> GPLGSMSGIALSRLAQERKAWRKDHPFGFVAVPTKNPDGTMNLMNWECAIPGKKGTPWEGGLFKLRMLFKDDYPSSPPKCKFEPPLFHPNVYPSGTVCLSILEEDKDWRPAITIKQILLGIQELLNEPNIQDPAQA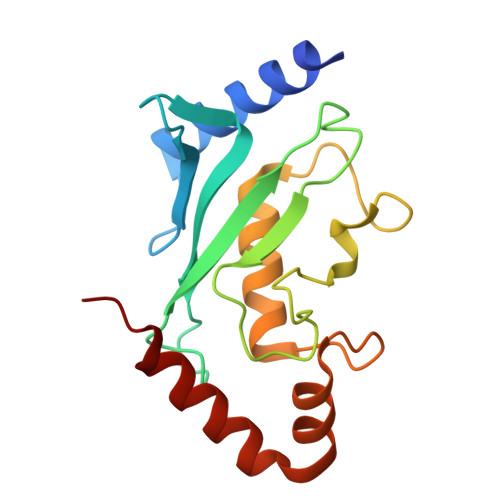EAYTIYCQNRVEYEKRVRAQAKKFAPS> MSFMDQIPGGGNYPKLPVECLPNFPIQPSLTFRGRNDSHKLKNFISEIMLNMSMISWPNDASRIVYCRRHLLNPAAQWANDFVQEQGILEITFDTFIQGLYQHFYKPPDINKIFNAITQLSEAKLGIERLNQRFRKIWDRMPPDFMTEKAAIMTYTRLLTKETYNIVRMHKPETLKDAMEEAYQTTALTERFFPGFELDADGDTIIGATTHLQEEYDSDYDSEDNLTQNGYVHTVRTRRSYNKPMSNHRNRRNNNPSREECIKNRLCFYCKKEGHRLNECRARKAVLTDLELESKDQQTPFIKTLPIVHYIAIPEMDNTAEKTIKIQNTKVKTLFDSGSPTSFIRRDIVELLKYEIYETPPLRFRGFVATKSAVTSEAVTIDLKINDLHITLAAYILDNMDYQLLIGNPILRR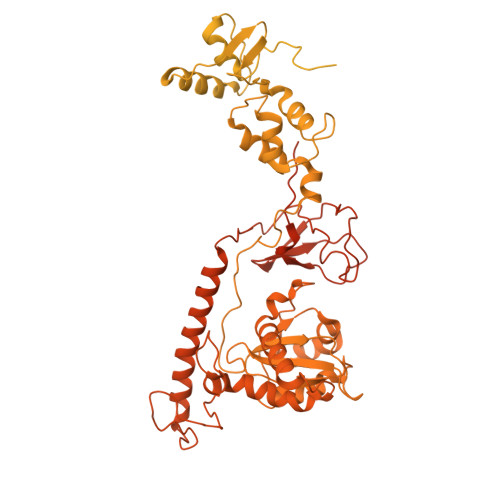YPKILHTVLNTRESPDSLKPKTYRSETVNNVRTYSAGNRGNPRNIKLSFAPTILEATDPKSAGNRGDSRTKTLSLATTTPAAIDPLTTLDNPGSTQSTFAQFPIPEEASILEEDGKYSNVVSTIQSVEPNATDHSNKDTFCTLPVWLQQKYREIIRNDLPPRPADINNIPVKHDIEIKPGARLPRLQPYHVTEKNEQEINKIVQKLLDNKFIVPSKSPCSSPVVLVPKKDGTFRLCVDYRTLNKATISDPFPLPRIDNLLSRIGNAQIFTTLDLHSGYHQIPMEPKDRYKTAFVTPSGKYEYTVMPFGLVNAPSTFARYMADTFRDLRFVNVYLDDILIFSESPEEHWKHLDTVLERLKNENLIVKKKKCKFASEETEFLGYSIGIQKIAPLQHKCAAIRDFPTPKTVKQAQRFLGMINYYRRFIPNCSKIAQPIQLFICDKSQWTEKQDKAIDKLKDALCNSPVLVPFNNKANYRLTTDASKDGIGAVLEEVDNKNKLVGVVGYFSKSLESAQKNYPAGELELLGIIKALHHFRYMLHGKHFTLRTDHISLLSLQNKNEPARRVQRWLDDLATYDFTLEYLAGPKNVVADAISRAVYTITPETSRPIDTESWKSYYKSDPLCSAVLIHMKELTQHNVTPEDMSAFRSYQKKLELSETFRKNYSLEDEMIYYQDRLVVPIKQQNAVMRLYHDHTLFGGHFGVTVTLAKISPIYYWPKLQHSIIQYIRTCVQCQLIKSHRPRLHGLLQPLPIAEGRWLDISMDFVTGLPPTSNNLNMILVVVDRFSKRAHFIATRKTLDATQLIDLLFRYIFSYHGFPRTITSDRDVRMTADKYQELTKRLGIKSTMSSANHPQTDGQSERTIQTLNRLLRAYASTNIQNWHVYLPQIEFVYNSTPTRTLGKSPFEIDLGYLPNTPAIKSDDEVNARSFTAVELAKHLKALTIQTKEQLEHAQIEMETNNNQRRKPLLLNIGDHVLVHRDAYFKKGAYMKVQQIYVGPFRVVKKINDNAYELDLNSHKKKHRVINVQFLKKFVYRPDAYPKNKPISSTERIKRAHEVTALIGIDTTHKTYLCHMQDVDPTLSVEYSEAEFCQIPERTRRSILANFRQLYETQDNPEREEDVVSQNEICQYDNTSP> MTGMSREEVESLIQEVLEVY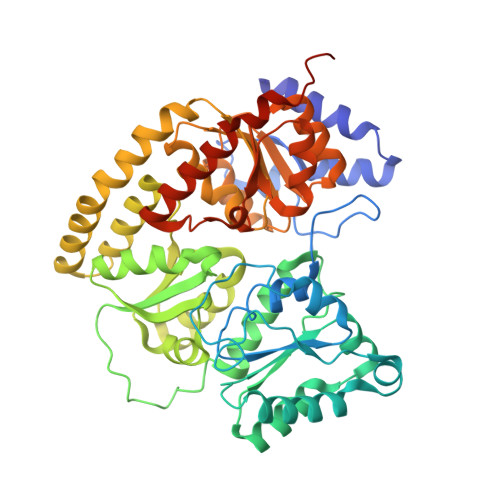PEKARKDRNKHLAVNDPAVTQSKKCIISNKKSQPGLMTIRGCAYAGSKGVVWGPIKDMIHISHGPVGCGQYSRAGRRNYYIGTTGVNAFVTMNFTSDFQEKDIVFGGDKKLAKLIDEVETLFPLNKGISVQSECPIGLIGDDIESVSKVKGAELSKTIVPVRCEGFRGVSQSLGHHIANDAVRDWVLGKRDEDTTFASTPYDVAIIGDYNIGGDAWSSRILLEEMGLRCVAQWSGDGSISEIELTPKVKLNLVHCYRSMNYISRHMEEKYGIPWMEYNFFGPTKTIESLRAIAAKFDESIQKKCEEVIAKYKPEWEAVVAKYRPRLEGKRVMLYIGGLRPRHVIGAYEDLGMEVVGTGYEFAHNDDYDRTMKEMGDSTLLYDDVTGYEFEEFVKRIKPDLIGSGIKEKFIFQKMGIPFRQMHSWDYSGPYHGFDGFAIFARDMDMTLNNPCWKKLQAPWEASEGAEKVAASA> GPMQQANLGDGVATARLLSRSDWGARLPKSVEHFQGPAPYVIIHHSYMPAVCYSTPDCMKSMRDMQDFHQLERGWNDIGYSFGIGGDGMIYTGRGFNVIGAHA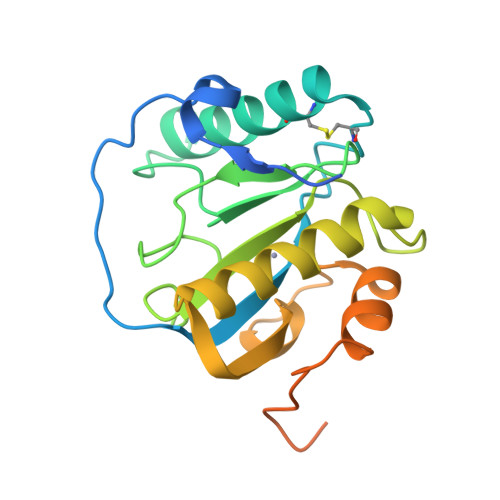PKYNDKSVGIVLIGDWRTELPPKQMLDAAKNLIAFGVFKGYIDPAYKLLGHRQVRDTECPGGRLFAEISSWPHFTHINDTEGVSSTTAPVVPHVHPQAAAPQKPHQSPPAAPKV>[2x]MQSTPLLQIQPHFHVEVIEPKQVYLLGEQANHALTGQLYCQILPLLNGQYTLEQIVEKLDGEVPPEYIDYVLERLAEKGYLTEAAPELSSEVAAFWSELGIAPPVAAEALRQPVTLTPVGNISEVTVAALTTALRDIGISVQTPTEAGSPTALNVVLTDDYLQPELAKINKQALESQQTWLLVKPVGSVLWLGPVFVPGKTGCWDCLAHRLRGNREVEASVLRQKQAQQQRNGQSGSVIGCLPTARATLPSTLQTGLQFAATEIAKWIVKYHVNATAPGTVFFPTLDGKIITLNHSILDLKSHILIKRSQCPTCGDPKILQHRGFE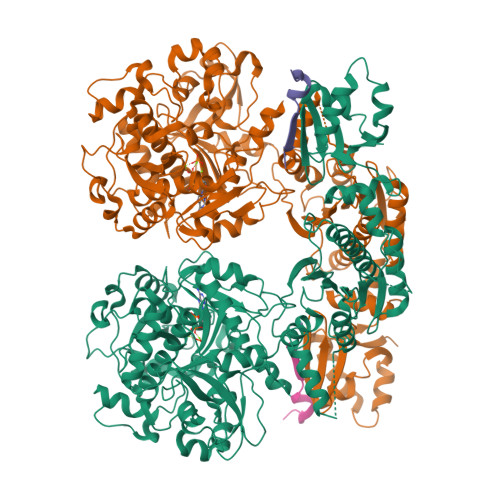PLKLESRPKQFTSDGGHRGTTPEQTVQKYQHLISPVTGVVTELVRITDPANPLVHTYRAGHSFGSATSLRGLRNTLKHKSSGKGKTDSQSKASGLCEAVERYSGIFQGDEPRKRATLAELGDLAIHPEQCLCFSDGQYANRETLNEQATVAHDWIPQRFDASQAIEWTPVWSLTEQTHKYLPTALCYYHYPLPPEHRFARGDSNGNAAGNTLEEAILQGFMELVERDGVALWWYNRLRRPAVDLGSFNEPYFVQLQQFYRENDRDLWVLDLTADLGIPAFAGVSNRKTGSSERLILGFGAHLDPTIAILRAVTEVNQIGLELDKVPDENLKSDATDWLITEKLADHPYLLPDTTQPLKTAQDYPKRWSDDIYTDVMTCVNIAQQAGLETLVIDQTRPDIGLNVVKVTVPGMRHFWSRFGEGRLYDVPVKLGWLDEPLTEAQMNPTPMPF;>[2x]MDKKNILPQQGQPVIRLTAGQLSSQLAELSEEALGDAGLEASKITACITFAAYDGELEHHHHHH>MHHHHHHENLYFQGMQEIIGASLVFLCNEKCEVLEDYGVVFDEKIVEIGDYHNLTLKYPHLKAQFFENSVLLPAFINAHTHFEFSNNKASFDYGSFSGWLGSVLNNGGAILENCQGAIQNAIMAQLKSGVGSVGAISNHLIEVNLLKESPLNAVVFLEFLGSSYSLEKLKAFEAKFKELKDLEDQKLKAALAVHAPYSVQKDMALSVIQLAKDSQSLLSTHFLESLEELEWVENSKGWFENFYQRFLKESNFTSLYEGANDYIDMFKDTHTLFVHNQFASLEALKRIKSQVKNAFLI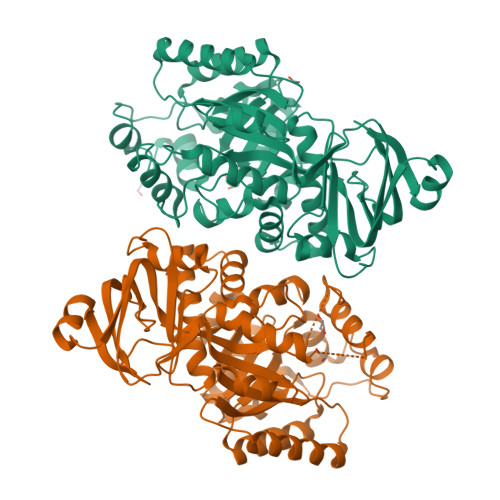TCPFSNRLLSGKALDLERVREAGLSVSVATDGLSSNISLSLLDELRAFLLSHNMPLLELAKIALLGATRHGAKALALNNGEIETNKRADLSVFGFNEKFTKEQAILQFLLHAKEVERLFLGGKRVI[4x]> GHMVSLDKAVIARLRKGGEEFEVLVDPYLARDLKEGKEVNFEDLLAAEEVFKDAKKGERASVDELRKIFGTDDVFEIARKIILEGEVQITAEQRREMLEAKRKQIIN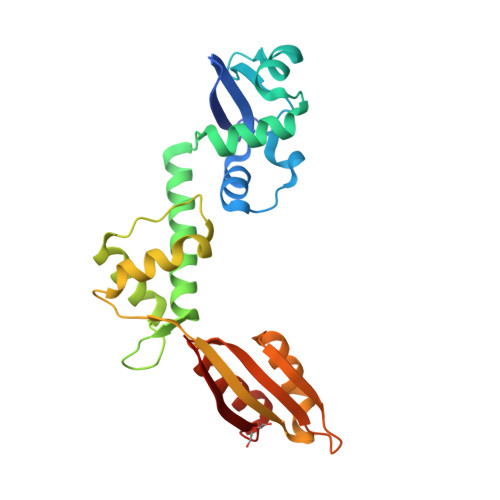FISRNTIDPRTNAPHPPSRIERALEEAKVHIDIFKSVEAQVKDIVKALKPILPLKFEEMEIAIKIPPEHTGRAISALYNFGGVTREEWQRDGSWICVMRIPSGMYGDLMDLLGKVAKGEALTKVLRRIG>ATPHINAEMGDFADVVLMPGDPLRAKYIAETFLEDAREVNNVRGMLGFTGTYKGRKISVMGHGMGIPSCSIYTKELITDFGVKKIIRVASCGAVLPHVKLRDVVIGMGACTDSKVNRIRFKDHDFAAIADFDMVRNAVDAAKALGIDARVGNLFSADLFYSPDGEMFDVMEKYGILGV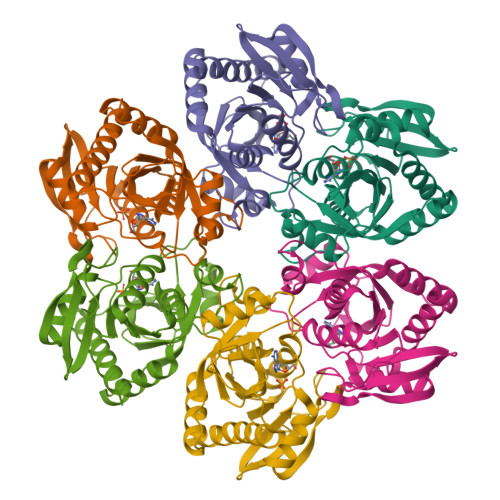EMEAAGIYGVAAEFGAKALTICTVSDHIRTHEQTTAAERQTTFNDMIKIALESVLLGDK[3x]3,5-bis(fluoranyl)-~{N}-oxidanyl-4-[(5-pyrimidin-2-yl-1,2,3,4-tetrazol-2-yl)methyl]benzamide | C13 H9 F2 N7 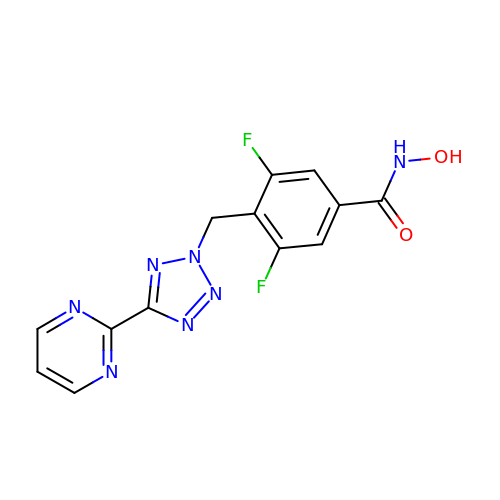O2 | IAJVLFQKWJCAML-UHFFFAOYSA-N> GAMKNEYLLLTPGPLSTSEAVREAMLKDWCTWDDEYNKDIVEVIRTKLVKLATKHSGYTSVLMQGSGTASVEATIGSAIGKE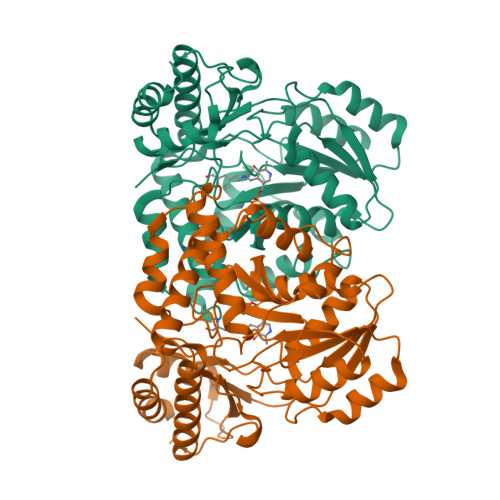GKLLVVDNGAYGARIAQIADYLNIPCHAVSPGETSQPHLNEVETALASDPAITHVAIVHCETTTGMLNPIEAFASAAKAHGKVVILDAMSSFGGIPIDIAELGIDFMISSANKCIQGVPGFGFVIAKKTELEKCQGQARSLSLDLYDQWHCMEVNHGKWRFTSPTHTVRAFYQALLELEQEGGIEARHNRYQTNQKTLVAGMRSLGFEPLLSDDLHSPIITSFYSPTHSDYQFKAFYTRLKEQGFVIYPGKVSNADCFRIGNIGEVYPADIERLIGAIEKAMYWQVA> MFRLTAASQKNLNSWYTKGTMRGGVPRIYYAWMRPGSFTRRRFEKMRNPFVDLETGTSLYFRDTRDSAEAIAHAADSKGIKGMDNAIDLYNEYRIVPDLYPEGFQWKHKLNTEYNQWRSNTWLTPDLIPKEHRGRFLCNFQLNIVAYDMRVVKFSPKDHRQWIYCVLYVGSGKGIAGWGRAVAPSTQEAKKEAIREAFSNIIAVDLEQEGPMYPVRVNADGVRVLLYPARRIVANFRVADILCAFGFQHAGCRINLKATNNPKSPTHTVEGVFEAVKALRSVSEIAASRGKVPHSLIYNIYPYLEEIRRRKGMMAMHPPGKDGLLMPDRVVDNRLPDHLKRGYYDDVYWKDFFAGSDEHLNEPRMGLRGDEMRRRLEEAQTSPAPTTAKDTRRRTLEDVLKRLGKTTRDLGSIPIVNPRVDVGLPTHIKRNYQLH;> MVFYSFVLVMKPRQRRFTSQALREIGVAVYSNGGLIRSITNEGIMRPYSRFRDADNTPLTYARYIILQLDMGEEEMGKVDKIIREHQDVLMALKLNNLERPVGIRSGNKELQAAYFPLDTFTRLEEEINWSPQTSADIYTQLEMNWKEFSRTRWSSFLRN;> MLRQSLLSLAKVYGAVPPLGAAQGHRLLHGKREREGSLFAVANDVKRDERLLRQQLNALLEEERMPMQARLQRNEAVSSHEAVPQTPLVDLPGVERRRDLPADPITRLFFQHKGDHALYYGTYDKPSVQDDDRVQIEKRVPRRREENLYTPIYDFCHRIREATEQRKRFVVVPSTIETRGCARVMHDHGLVAGFRDFHNDRAFAVELKYFQGDSTINVIEPCSYDGRTEFEWSPKMMRRLLNTHGIHNRLVVYICRTADNRIIDHIHAVKENIGGRGLMMVH;> MMRKSVTFLRRGKPRPRAGMFPDKYRRVPMLLKPQQGGQQYFNHFLIRSTNDRLTQQDVDNASGQAHSFISPQLPQMDWRNMSARSSEESIREEMRQLAENDVMQHQRVFNERMWYEKEEEHRMKARSCPEETSEHAISNDGAVPPPRVLGGDYFKTRFGYSLVKNSEMTQGPVDYSQLDMWGEMPRYTSDMVFLYLVSRRRNTYAVAYTYEGKRILNTYTAGNRGLKGGDRGFRSEGSTDNGHQVTSMYLNDLLPKLREMRASEGRPMGRGEKVELVVRVMGFYNGRQGAVRAVQDRANEFHVRYFEDITPFPLNGPKMPRGVFK;> MFVRSFCFLRKYGSKSKTPDLKTSFTKTTNFRKAEKISITTTDGEIVKGRGKIRRRTHSALKEAIGAMEHPAIWLWYPWRMNPEPPTPHMPQRRALKNVHGAVFNDLTPVQKKRQEQMLYGVNIPETRQMKFEEQHPLLAGALRKLEGQPKGFPFWYRKYPTRRHAYEYRFSIPVEMLDGYNDDVKKALSKGMMSIQEKQFAQEAMYMERYAEHDFDTTSPAVLAVKRALKCRVLRNHLLTNPHNNIIKTVLANTERKLNHALRRLRKVDFKKYWEIIRDHDVQDILQPPNLVTYRQGSYWKYDWNAGLAISTNLADVMDPRGLNGCVETGRSRSEVARDLGLSYTRPLHENEKKQLSHQAVYYERLAKFKMEQPEAARAMERERFVRKFSGMFVKMDIRSGAPDFPSTYRRLLGTKVVRWASKRHGPN;> MQVTETVLARAVIKRRSPQLWGAPGAPIIRMRGHHVVWKFQSYDLVVEHTHKRRNSDIRLLHYLGKHCPHPQKSLWSPDTPVAQDRHLFMLTTVDIDAFKYWFGVKRCRLSMKPWALLAKAGLLPPSLTQNSKIMPKPLFDKESLMRYYLANRKDEDVMAREKYLNYENSMVKTEEERAAERPVAPYL;> MLRRSLLAFPWWNFQTEHRQRCVLMYGGARTKNTHNANHRVFIKKYKRNAFPNRTRHHWAVSMTGVLSQRPRRMPWPYDLTSLIFNQPRQGSDKIGYVVGTSMLKTAVVATNHMVYYPKFNQRVSRTKRFFAHDEDLACVEGDLVHIKQCRKISKYKHYYVFSILEPNVEGRERLKLGLKAVPPPLFGYPVSRRIVKLNLTSTEGTQEKLAAAIQEHVQDAYRFSGPTPDQPRNRLADPVTFEDANNMIAPNAPAAAALDASDSPPLLDRGEYTEVEQDTRNKKGDDYWMNLQPKEKYDFKSFKKSPRPLEDQVDPRLIDGKYDIPTTASENLYFQ;> MNRTGGSIYAHALSQFAVCRQPWNEYIGLLTKQDSTPYHTEPQEKPAYRGRKQGREGWLFGQQVQLHYHRFPDEQLITNLSRWRTGETVGDIAMQQFRNAQPFDIEDKDPQGVQRPSPEVYMKLNYKNPATISRFLTRTGHMYPADILPLNPEAVVKLRVAKAQAIRIGLYPRFGNPFWFRSQKFRPKAYQENYDPTTYSTKRTVEHFAYNWVQTDRIRRYFRELEAVHTSGSASARGSGGGTTAEHKQQDQFYSPENQPISLHRNNISYMEDVGRSVKNPTVPGLMSTKGMKKKFHNLYSSTSTKRMGFSNPTLGIKKV;> MLRRAYIQRRYPFNKRGPREHKSWKHHVLTEPPKPLQWRDPKVWTRDLSVMKSFDAPQWDLWQSRPRSEDMDEALQPFMDMPKSLKDRRYDIPWWANPFGAWYLQNILSLELLKLKSKTNAEKIATYRSYMRSLASGKDNTMSDDDVIRNIIKERWKTLEFGDRNAGYPCTFGDYIQFLNEWFKSLDEEGMQRLREHFDRRIRPLLAVMSPVDILWLEALTQNSPHNKEQLQRKIAFQTSLGTPEFFDMSKRLRYEINEDYKVRDELGPELFALWSKAPERWPPERLSKMYGLDFTLVRKILVWHHFKACYDACVEPDWSLPKRLFALEWIRDVRARKHGLFYGKMRFAEQKITFYSDRFLFRDLVNRREASYANVWEMDDPYRFLQTEQDYEDYWGDNYDVYRRMFPEMIGRTGEPVQQYGQMPIWAGPHRQHANKSEHNWMFAEIGVNVGHEALKKLELDPTNEKRRRFVIRQPDGTLRSAKMSEMRAWYWKEEWADFRFWAPQMEWGIENTPSQEQYQEHVPDTTDADFRKQRRIQSRPVKWFYESHYTRTGSFAGFQPLRFMQRRTEREVRWPDVINAAVQIQKRKPAAYIFKAIPEL;> MRQCVVRRYKMPKNMGVAPRFDTWNEKYEPWEHMKRMGRLVGTGFYIPPEWYNHFRMFPPINHNFQQEKTLNPHNASEPTQDDTSTLSPERVALRDELARKSRLVASEGMRYYNIFWVRKPLDTMEKEYYELKRRGVDHGEAIRKVLQGFYSGLAVKKRVAAIQAEEAKLTGRFITMREATVVLGVLAKLHKEQLTPHQVSLLAKEQGETTQSGAKLTAIVSRTQPHVNKEASSPATSEAVGSSTEESLSADALASMLSEDGEQSAVGTRYQVEVKETANDSVRQLREKAEDQTGFPDWYTGESPTYSGTS;> MMRSSSFCRRQIRPYYNLPSKSEHGRKMTGFLTPYRHWMWKQNELWRNVHEAQFEHLRRVYKRQWLESFRVNADEYIYKYNITKAAQLAQWECEMKEQEKKRIEARQMMDGRQALKKKHLDLLREFHERQFFFWYERASERLQNMNLINYVPHAQLREHIDKELDKYVAGKNEPYPLNFVGQMPFLEDGDGNIVEVPESLLSNHMAEHPDSTAKPHEPHTSSSISEAAAFEERMLRAMVSAKEEDLKEWLGDDSRALSETIDDISREEEEREADIRVARSMEETDAEREVSRRAYIERGKTGSRSIFRPPTVSEGAGGTPSAPAGDANTPMRRRKKGKLDRVHALQAHQDELLAKLSSQGLKEGVDASSVPERGKIVQSRGRIRDKAVIPTHEVLMQKPELAAGSTPGARIQTKDMVDKMYHRGKYKKSGSGDKSDGEDL;> MLRCARVALRADPLNGGSSMTLGSKGSKLSPEPHRRRMPWTAAKEYVPGVVLNARDKMVLDGVQLLDIESIDRASQLDPLEVLRAVVATREYNISTGKNIFQLASQATYNGRGQRFYRKEWQEGTYDKYVTLSAIDFDRDGNKGTAYGYITFHGETTTRPVQVDFADVPGWYMDFVEERAVPFTGIVPPPPSIGTDVPVDPHSYRLKAYPYYDAPNPPEFVERLLKDRGVLPDTPTETADVDKDPTTSDGSVHYDGK;> MRAGCVACSRIPKLGIAALGSTTTSMQATCQETQELRCATTQMAPAVIFPLPPPLRGSYIDRKPTAASFNEHHATASFRHHMIASADVSHRPRHFYFASGTRNDTGTRSVKEGERKQLKQQTNVEVDSVAYGDQLDELSARWAAKFYGQVTFGPRNYPYPSSRWLARRFQMKKHRIIKRFRFRRYKLAAVANLPFAKMIRVGMLPELKSSKTKRGDVVDPTLSGQLVSAVKNTGEKRKGQRTRPKSKYQV;> MLKRTLTVLDQTYGPHKSYKYTYMPDPRKLAPIETTQRSEIVPQSIRPPTSYVPNHETFLERADIHRLRPTSDFKASFKDWNDLFTCDKRQLRVRGIPRMTRDAIRTAVQAFQNGNPPERFDTKEEWLYYKQFKTVDYSYRVIPELPEKYRPHQSGIDQAPLPDYREINKMPQWAECEERRQSKKTV;> MLRCTVVGHHRSGKARAFVFRDPSLRMMRAGSGYQQLRRMGMPMQVGMGWRKVDSFHANTQYQHAWPLLSHDDLGNSDQSNNTKNIMYSMYMPKRNKGTAPWFRGADTYSVKYCEQGRYEYQRYLMINRFPSEYKKHFLSFLSNIRMSSGSATIPQEALHWLLRMIVDNFNPQHVHYIAAMKTLQSAGELDMARDVWKIMERQQTWPCTATICAYLDVCVEAGEKTWAMEAWNRYCTELKFLEPGEVDPKPISRVPFSLTREELLYLPKWKKHFDHDPNLDVMDLNRFNRTREVYLRMAQVMLAGGERNAFQHFFTKLEEAMLNKPTPVPEPPNPHLVRRPRWAPYEHCKSVHHSPWRLQNNGRALALGPPVTIEDEMQSRFFSNDQFLVHSVKEVLRIVLQEHKRAHPTECTRCKTEAFFYKTKDADETLKFCDDLIERLFASLGVRLSNLNTSSLLSTILEVFRVVGKESGAALLQRANEFLERKASLGDAEGSRENLTASNYLQVLSGFADESAFVYNTKKDGTCQYKTGFDPRTTMRHLADVVQEIAGNPHVTWAADMHLQVVETMVGCGTMKANDYFVRNVLRQFSWDSRFLEALYVEYRRQDDVDMWAELTKRALVWTARYNAPASERLRRLIEDDYDTIRVQTRTFRELAVFQFRDVEERRHSRDVVNELPNPWYDYVAHALPFPDRDAGYPDEYGDLGQWRAPGGPGSPVRGPGYYAPPMEGEHQRGYTAEWRDLRNPMRPPEFPTPWERKYRQYARGQHPSYDMVYAGPMPEIFPMRRDFRKPTRWDFHDIEKQGKYRTSGPY;> MRKFCHFMANCWNSARSHATYGAVPLTHSQVTSVYATDGGKVDELGLLELVEERIFSWKLNKWEMRIPPNLPNDQKELIRQEQENLKQILSEWRKCFGALNADILQISSLTGVPKDVVREKNRTWLQEEVAKLRWMGEVNKAALLRDAFMRLEAFGSRDFMFMERLCCIYGLARQGTFDEAFTNYITEDPVTNDIFVDERNPFKELVAHIVRNYSQIDIIYDFLGFNYSEGYRSSLRRYMEYLQCKTAENVRASGRLVTGDKGEHNILFDYCVSRESLVSGDSCQGIIDFLYINGNDVTLIIIASDNPWLRNRQLPHRRQMEGIARRVCFVLGIPPSEVRIRNLLLPPTYLDKGSIVRLNDIVFRLSNEQSNLLIPWLTNYNKELDPKDVDYTALAKTTNEEEWLTL;> MRCSCAFLDKSVFAAKRRVIVPIHPTPNFPAHFIKSAFTTDPLKEKQKARFSSGGEAMREVQDIPKNLEGERSRRDLASRGDTEFQALVEFIEGASYDQLISGRRFKKVYDVLSENDDMFIWLCHTAMSVLNPGDMRSRLIYNHLRILAESVASGEMTQRTAFRFFESAVRSPAYREIAKRQLEGGAATRLAGISAAADVMRRMGLTRRPMSSYFELYQRIVERSEAMTPWGFPPLFQFEERLSLEPRLKFFSRASQQSLERRRRGHVMTPHTTLHGRRIFWIPPTWNRAGRFLGPHVTLYPGMTPD;> MRRFCTARVSSYVKRAPLLLPRGGRRWRSGAGTTADGGGEKEYIADSFESTAGSNAYAAMELAAEARREIHELWLSAETALEREKRVQQVAALIEKYKLDPSTPREADVSRGLGDAFDRLLLLCLPLGKTDAKGTDNLERLMHLAGRNGRELSVRTIQHLFARTDSFAEALAVFYTMRRCHVAMNMEAYYSMLYSLQRLEEEGWGQHFRNEYEENGAPSEQAMDFIVKGISNALLPENKPWLGRVMFQDRNVPDRRYDTRDFDELDTAWTQRYKSGTPAGAH;> MLHGTPVRRASLRYRRPYWMMFLKGVDNWKIYTVIQQPDHQRTEMLYQAWLGGLDRPYTRPKCMANQPLWLSKKRHMLRKERLDGPETPLEKYVLEWHKKFHSFQGTERPTPDDLHTALDLVERPLDLSYALQLLGQCRNLNNIRFAKETFLVFLEACLRVGRRDCAEYALEHAEPLGFWFIDEDHRRYLQGEQTWYKLSPLDNLYYPVEENAKLNEGRKPITRLSPATESPGSGTAISDGEPSTDVEGETTVDDEIAQLEAELAALEREGGGK;> MFSESLCILSRRFRYNTKFPALVSYNKLPWEVVNHETPQFHMHVAPHYEQLLTLAASSPVPHIIGSKHIDVPREHRLRLLPGMLYLLDGDTLPGEFTINRVLDPTALQYYGRLSSQIVTVEAVRMLVPDDLRLLCNCITFKGPLHLPVAPYASLASLRGASQGGTTGSETGSNCFTLYHFVRPNRPPKELQLEKYYIHAPCVAPLSEFASNSDERGNWRPRLQAPKRTRRATPLPAYRPPQSYLMGLAERLAVVPGGCFGRRSLMWGHWF;> MRRGALSLLKAGLLGHYQQEAFEARKRFEESTTYPGPIRAATPGDTRFYSGSLESILHDTDRHYWRAVTDDPRVQHLIPLRIRFKIFTWVTSGWEQRMQVVQIMAPKDSTIAQVKDLVIVENQSPYLCVSSFHLAIDGKELDPQKTLGEYGITEQSQIDAIEQNDHLLHRDDERPRDWTVDEITAEDVKRSPYKEMEMQPLQNLAPRYEARPKGYFGRTYYSGMKQSS;> MLRRSILFRMKYADLELTTRGEFPHGMKEPAFVKKLDQNIPWYFSTYRSMYHWPITGDNWSDLNEAEKHHDLHMFYTLAWWKLGEGIFGVDEDS;> MFFRFHSTTLQTCLTSGVARSSVAVAVPLRAGCTRREMSSGGDGVLEGAMHKPGESGLQAGSSTTIAGKETWSQFSTKMRYGRRRIRVIDVAAKMSYEYQMLRKMCKRRPAMRQWAVRDDFCDMNPGVVIMSPSMQAAFMKVFRMKEKGLIRQCLRDIVPVIEYRNREEPARLPTNPADMIPEGEPDTLNQKKRELFERREKGENFADLRLHDKRSQAKLRFRIRQRLLKFQRQLAVANAIASRSVLYSTNDAIGYFLFRGAAMYAGMHRVFFELSKQLPHFVPKTMLDFGAGTGTAILVAKEVYDPGSLAYPLYRSLRQTMQGNDSSRTHQLSELRYDLKRLQRNNEEKKKVRFMAVAALLERGEVDPADLPEDLKREIAEVATAAATAKKDRLVREAHARYRDVVDGTEWESGDPLGEVRASTEDPEDVIDGEQGDGGDDGEAAKGRPKTWWEKLIDVENETARTRAARRLRPLQEVTAVEPSPGMMEIGTMVLHDDVPNVTWKRYLLPEDEAIQHDLVVAAYSLSEIATSENRRRIVQQLWKMTKGVLVFVEFANLNNFNILMEARDWILEEKDVGLWDWQPTIVAPCPHEHRCPLRHCKTGVKRKRMRICSTEAHYRSTFVEVWARHMPLKVGIEPISYLILARNELVPERAERRREQLKKAEEMKRRERDVKQQQLHEASLAVKDVVFERLSDEALHRVQSSVPQPLTDIDEVREASTSATSTSLLKDLKDGATSTGEIGHMPTDVPRLVKTGNTRHNRLIFPLQFPPATHKFNRAFVDAGYQRQRAITPAEMLVVRQEVEQLQQRVMRAAPKYLRVVRDPRCHGKVQADFCTPEGDLVSGRVYRRFYGDRNRVSAHSTMRWQHIGGWKLLKRIRRGSLFPHNVPLYAVTKHAQIDFPNTLLDTKHSTVEQTAMQYNDPMSLVEMPDDGLTREELKQKRRLQRDVELQKKVEEKLEDIFGVNAKDWKTDDLGGGRLDARREISEQQWADAVRRAKIRTVQHTKNALPFAAKKRAAQRALQVRRRNVRLEMSGNRRR;> MLTPTRRLPKALSPYAQALRHVALRGATAFGPGAKEMELDMLRKGTLPADYRPPVQGRWDDTIERWAYAWQFPAEEEQDDITKSVERNASGMQALLEIGNKLLRSPPSPEPLSGKASKLYPPVGDMSSGNTALLPPNPTYDVLEQDVSELMAEDAVVVTSQPRLRAEELSAKYNVPMAYIDDSSEASNASKSLALVMEDVGLEFTEDGLTVVISALSRQGYGTIGRAIFDFASAMGLGPSAEMYRALMKYASRRGDVNESMALIEEMKGNGITPRIGNWHELMYTFYKAKDYPAVSQIVDNMKMYANIEPNEVTFVLQLKALAKDNSQLNSLPEAIQLFDQMENVYGFIASRPHYDAMMFHLSQSPRPEMRLRCEELAHKMELMGIVWNANTYLNLIRSAQVVGDVAAVEKYLSRMREEGIPASIGHLTWAVQAHVQSMIRIDYDALKEKDESPLPTWLEHLETCFGIYELVVRRGWVMQLPFVNALLRLTCQATILSMERTPDEAETIGRFEEQANKIWNHTFDEWQLQKDVYSYECYIALLAHQQRIDEAEKLFQEMILKKDLSPSRRTYHCMIFMHLSSGEEGGTARALRYLEAMERAGIQVRPSLLKKIVRVNNAAGYKRDMKRRARRIMQAREEYLARKEEGVSFGEGGKEGASNQRADVDAEGNSILEPLAVSPTSTLAWWEKWKRETVSKHELFTEEGADGTPKGETFEEKNEALRMMGITSSFQTKDLVPQPDRQKLLPLIRREEGEIAGSLWAMDGGELSYPKDGGGPQGWGVRLWRERQLVKREYQKVLDGYRPVPQLSTLGNSVRTAGDQLDIERSGAQTPGELSDYRNFPDNRFDGGQLKPESEAAPAVPFSAELVWQGEANDKLSPYKSDEEIALENDNTFFSSLSKETEGKLSIAVKAMQNKEENSVDVRGKGVTRRSKFDYLEKWRDMYRHGTLEVPEGPTLNFGRTPDDHKETMAALVRGWYQRNRKEPASEEELKRWRVDEQRSSETSASRAALKKRKQVRSRHRNK;> MLRGWHPNSSAMQVGMRHITIGGRHSRGGFRQPLGKHPQVKQGTVEGVPRRIPGTTKVTYTNKKGRTFSFSVPVSELTHPQVTLESAAGTWREMDTSFCELGDIEDDMPSPVDECLRGGSSLDKRLIQEVRERFVSFCREYVLMDTSGMKSTILSTELNAGPDYEHYDRRLRRKRHWLAIRHRFEDVRYVIWPDVVEETARGDSAQADVSLTNPSLTAGEMLEALLWLDAASTFCVRKVHPSDLGDKSEFLPLDLQREVEVVACHARRDLDFFDPSATSLEQFTACAALCVNHRVPFSLFFPAQDVCGDASVSTGQCIVANAPSPHTALGAVRIMALISEGSGSDIGKTIMFSDAFGAVTRFGILRGLSRVMSVEAFGCKDALENVNESELCIILHFCAEVREQNAAFFRRYEASEEDSDPQQVSFLAKYQQLSQIALARCKRLLYHPDSPRAQVMSEDGYIPLVELQRHAEGTNKAALIHYNLGIRSAQGMRRVALGAQSSARLAELVSRLEEASARVSGNTLVNDLVHHLSHKAAAGKMSLTLREVNTLLPLLSRMRRESPNGALDARFDRVFNAIDTAIGAAMRHNCTLDELLDLAEGLAACEMVPSALKQVEMVLIRSVMMHECSPMHLRRMLQAMFTLMRTSVPQVLLQSVASRVADYIKEASHMDSSSSNGGGDEKVKNHEECEQLLELLVVLGKCGYGALPGLVTIYWEAQLIDSMQLNPRLRCSYASLLASAAFALKKHDKRAWEGLADESHRLFMEYTRCNKENDIGRFAECVTGLAVLTQIKDNTNSSDVAFLKEYLSATSLELKSCEVIRVQELTDLLGRTLEWSEALGVVAPDVVIQLEKALFVMLENVSHTAPGVGIPDELVTAACCLVDMSSASLELRKAAAGVVGGAIVHAEEALETLRSGAPTQVRPGHSFDVAALASAERENVYKNSILQYCAALQRSGMSTHVEELWS;> MRHTIPFFRRSAFVPAPGSSLLNPRSQRAKVRRMVAAQKAQGENFERQALYAELGGSPSARAPRSKGERSKEATRRVGCEVAERAKHMTDAEWEGVPVDEKHAFAKYMHKVLQEHPTETTEQQRRRYFETTMADVFELDPRKTVRDEYERVKLGLPVHLKNPQYSLGVSQAVYDAADASLFDPENVHRLENAMTHVKQVFADYVHKKREGVSTEAERRMLANLTAELNLETQKHLANMFKYAEMRLRQVKLEERHHQLAEIERLRRMAQQRGGVKGRKGGSRKMSRMERLKRVINRAVGLDIAVAETVLTEMQAQEEFLQFCEVFARLTLGSGFKHTGKDENLSAYIESLRKLYSMDAATLSTLDVVQYYSSKEGAHPVDWAKRWYERALLLPLQSTPEYQKLLQIQQRDESTVKHIKETAGTGHAFACEAEAEVARIKTQKVVNLVEKMFMDPKDKRLESLHEKRLRYLAHMQMERQIRCVRENAKLFDGVENMPEAAQCRELYEKIMEKKTAQCNMTSPPEGEGSAIQSAKTEGDHCEVGPGMFNVYDDAEASSLFEKIREITLRVIRDRRVQSAAATKARMLNRIIRSLKGGERSIAEELRALHQQRKEKMTMRILGIIENDVKTEMEWLQNMEEAERPPLLPIPENMSYVSAADVQAWRELREDDERKAANPFERRRRTFQPELLGQAWSVPNKPLLFWGTGVSAVQQALRHVAEDAERKRQGLLLAPPYPCAENPWGWRLAKDILDDNN;> MYKKALHSFFLKVHPDFFHHNRSQQTVNESSVARLNELLSWAKAFKSGHLQPPPSSSFTLTFYRKPDDNMGNGETRREGSGSPVSSLVGRSMGDGSLSPTIIQSTFELPSNFAPSDNHRGTVERAVNKFLRDLLRRAACIDSVTESISEAEDATAARAEAKPLRRRPRGSQHRGAPTGPKSLLDEAVESMTVQWSLTPAPTLQELIEADQILFSRDLSPLQSAAALSTLQRHLGELNYSAWESMPVIVSNQFSIGDLTGTITIPWDFTPEQFHSFMAHNEKGVARCREVAIQYASTIEQLIAELCTALELDDILVSCSHQDALRLMELLHRNRELLIQYGLSKLTLEVGNRHATRANGVVIINCSLTSEQLRPWLKAISPKLPLQQRLYELSKQMLESTLWHLKEFRTMVEPGGVDAFSNDCTYAERLQWSKELFRIGPSLAPWDWSEMTFVLSPDVDIDWANGLLALPYNFDGDALVRYVEEVQQEAKSRKREELLAASAMQREEEERRRKQQHDEELMVECQEKGERSGDDSPTVAERMRHLYRQTNPHMDEYLASSNSRVDTLPVERPLSHAVTFNSDAEAEDQLKWEGFYAEPYVDQAPTSDIDDMAHTFMLTNRWHREEAAKKMLDQLRGTYGKKSRRFEYQKMGDVLEINNAKVQPKGFPTLTRGIKPGC;> MLSHAVPRLRLAAAAVKAAEWYAAENRRKQKGGDVIREKVDCTAPLWFDDTEQNLLAREQHVRSPAYRELHRPALTNAAMGLYGGEPGFEKAHRVWVDPDRPHIKHIYNQTALARNLRYARYGYFKRDMHLLDVDKLVRHARLLPTPGRLLTDFLYQRVPLPDKSCAALIRYQRQQIEMLEVWGRHASFQCAVEMFERMIVTNIPPVEVGVETHGEMVLCAAACGKWEEGWNVYANRARELEKESPESFILNTFFFDALLTLCVAAGRVSEGIDTLEEVIKRNLRPRGTMLNKAMILYSILGEQMSKHEASRATSEGERSYLCEPEEVEKMGLEVWSLFDFYQLPRTTASIEAYMRMCCAFNKPTLVLKAQGFADASDIRLSIECFHWLVYAIRGVAGFGDYVMDVLSQLRPRGLTPDFVLFTLSFMYCALQRDGELALAIFDQHFVHQNMNPTPEMVLLFIQACSNCEEPTAVMLERSETLIKRLEAVGSSVDLISPIYDQFLELCAHLGAVASGFSALKRIVGFGKPLTTRMINSLLLANSNAISSNGSLSMTEELVGFFTLLKIRPNADTEICVNLCRDAFGESPVVNDFIKVIGESLQGDSEKGEAPQYDEDIPVIQVPPHELRQLRTEWKLSPRDIVLRRFGQHTKPPGKAALDVGSMRGSVIPFGRSPGEQLV;> MMHRTAARLRMPRKPTPYVRKFLEGCPLPETLVDDIAGANLKSMAPFFTTAPRYIVAAESRLSKLFFHHALYPAGGARRPCRVLIVRGGRSVREPSFTINTGGGRGEVGGGSRGYRDPARRAYFYARPSTVGPFYSGNGGVSSNVAKCHSGVGSEGAGLVKRASVDGLLSPLCGVIEAHFAVGGTCNDAVATEGDGTESLTKGGEKLCVTLAGLLSGGHGGLMMDDGNCASNVRAAKRVARLLHDAAHHLSSFFYVHTQLPDSALFVSRPEASIASDGKGDGLLPSHLAREKDNDGRPSVEGVAVFRLAGGLEPTVHFAVGAPLSVLQRGVDGTASRGEKNSAEEGLNSAASTTVLPFGHIQCLLRVRTRGGKHCAAGKEGSEGTSNTPWCNTAGNDDITSNFAASGPQIAGGIVEPWKLGVSLDPKVPFFMRTLTEKRPSFSCGEGYLGTCSRSGDVDGNTVNDVSSSSGGSRTRAPGEVHMNHLLVRNDCETYLLPQRELLLSFHVPEEAEAMCKEQNEERMRRQAALGYGSPSHVFAEGPRTFARVLHGMKANLAAVEEASSTFRQGAAEGISPQVNGGSTTSGSSRVYEVRALPGDVVFVPRGWKYSVERIVGTAIIDAVAASTASPREALRAVFRTAPDPPLPQDVVRCDEGHAGAGEMPGGDSSNAEIVGVEVDAFVLCYKPYPVLSNAQASTYVAANYVHSGIDDFYAKGGNDVYHKYT;> MTGPTRALFLSSGINLGRLRLAEQFSSMNGWQSKEDPAFDAYVKERRRKENYEAFDQRVERGYAAAAKLHKAEIQNAVKRRLKSSGAKFTAETLREMSSAVTERLAWLRDVWAQIDADYRSGDSARQETAAQEISAALRGEPNDYMRWVYETKRELRFAGPVGRRAIQEELQAAELPEVLDEEVNRYHDLKLNMMEIEREVKAKYGVAGQQHWAELQAAKDEEYIQKLDEAAEVYKQLLDQSARLDESRRSELQRSYVERVHQAQVRFKAAMELEGQREQLIEAHQAMKEERMRTEREKRRQLLREAAELRAQGKKSADVLTALKERQLDANAKRQAEYELKECEDILKRKSEMLDMIAHFKHDVEEREGREMLQRQKSDEERQVNVFGFYEEVGVEDGLSISSEGTTSQGGSSGLGTVSTSTSCAKSADSNSSAQPSQKLRKEELWKVINADTYEDPFRTVHQARLDAVKTYDPAYARTFPLNLVLGRKYSRQGAGEMAAGNETDKQILQKGNNILYSFQWGLNNGTVHDLDADGGTDYFMDGAFHVRDKETGDIDWRYEKKRGGPVFRGPKFYRLGAQREAADPGERAMDPTPYTSTPREHKWRSS;> MPSASSGYTFADFLRRLERSPDSHMAPLYHEHRELFVRRHDMFARVISSVTWSKGVALVAAAGYTQAVNVTIYRALLARMLLHNRHVRQCGAGSVVPWSAALRTYSEAIATHGNAVPTRMTLSALRLCTPARQWVAAISLLMLSQANDKLTLPMLIDAAGCCATPAAWEKAMALLGRFHAQSLQVLPDSIQSLRPVGTSASTVDAAAHALLPRSEGPTPEQKHILTVINKVVSAVPWQVALSNEMCRSYLTHLVASTTLRPTEKTASLTTAVQQLPWEAFVTLMKTVTATVQEGSQGVLGSRSTPQLPPPQDGMERGDVAKSLLSNSIIREGVNLLQSEPETAIPFITTILYKLPSAEAAALFLSEATSAYRNSSSAVVAAAIRHPVVVGALLKRCADSNSWYLAASIFKSTSPTAIPCDVASDLVIQMRRANQAPLVVDVLQKYIVPSRTKLTEEAIEAALLCVLVHNRALAKASAVVAGTSPDNRTGKPNGIGVANGVHWISALSWATDLLEEGVESRILQTGTTPSVGGVNHEDPTVLLRKKTLSPRILSLLIYICVNAGSPRGGLFALGYARTVSKTELELSEEITALLYCMMYDRPREAESIIQHAVKKHGEYKGKYLGRLLVASQEAKGSALRNQT;>MRRLSVSFLPFHLIVTTQRRQFGGNSKDGHKGEDKPIERVGEVPPTGPHPFNITSGAEGQISNQQRKAHDAITQLFRDDAQRKALYQKPGRTIGAQTTTAAISTPPNEDEFEGLQPISGDAEPSSITAVEAVEQELLDDAFLYFPPAQQSASGSVATTATNELYVPGQQIIPPGLTRYRVDVQYQGNDFDGWWKSTTRQLFRREVGLDGSITRVPVAEPGTIGNAAGASRGETMGSRYHARTVLEEALAVALDVNTVRVVAGVIPEVGVSVRRLCCHVDVPSHIELQPRTVIQRATMWMEKRQQPLAILSYRRCKNQDFHARHSGLRRVYVYRILNRVAPPLFDAGLQWHVDRHLDVDRMKRFAKALEGTKDFGYFADPKMANALRRAAMSPGGFSTGAVTEENFQPKATGESHRVTRGKAPKVTMEKGPSNLDRAAALPTFNEYGQRVVQPGAHGKEYYRVATNLPTVRTVDRLDVVRQDDEVLIWFVGRSFLRHQIRNMVSVLKAAGHGLWNDLELQQALQSGFEPSRHRFKRERFPTAPAYGLTLWDVEYPDQHRDDYVQFVDSGPYEQVNIARDI[2x];> MKRYRSSVVTRLVRAITLRPDATVDPERYPLGYVPLDGSESVDSVWSLVKSGAFVAPLSKIETIHRAHVGIRYLTQSEYPALSSIDVVGLQTRLKELCSRLLIRRDFWVLDDYNDPELNSSFGIQNMYFDNFKWSQVLWRRFQQYVEEYFPVAEHTHLTYDEYLQLLRSFSHFEQGAKLLPLLPKRYRIHPPFGVPALSRIDMEPLLLYSQWLKNFRGPLKLDAALVIRSGCGAAVFATKLNGVPIVRGVDPNPRAVMSCRKDAQRMGRRFDSISFRVGEMFPDKDDGNGVPNSRKYDIIVFYPDQGCYNLFFTNAIGEYAPVLTGFAGTLEHFFEEAGDYLSDSGVIVLCCTNVYSILKPTEPHPIEYEIKVNRRWVLLDYYDMPVRGKGTLSHTPTDHHYRIPMEMRKCMRSELWVLHKMTSIAHFAHIHNIPGAQPPSCVVSHWRNKAIGKLRRAVLKGQVESSGGDWDDYKKRLVHLLQEQSENDEDDKAQAIRMAMDPNYPKELADRARAAIEKNMDTDKAFHNNVAKAFGDISPRERFDAYLSCYRL;> MKRIVVPHRWSEMNRVEHPPLMMKQLFQGVCGGLRWLETKSLAQYLAVRAIEEGYPSTPGVRKALHVKRAPLQKRRVVQRSTKSATAACSLPTTAAPAQLPLTSSGDALTVTGGLSLQVTKQKRLVSYDVLDCTLGSGYHAGAVLENGGPYTRVVALDCDHDAMHAARDLVEEFGGDRFRFYCCKMSEAKAMFGERSFDAIMIDGGVSDTQLEDPERGFLLDDEGGHRLDMRFGPQMGVGALEYLNTVSQHTLVSSLLAYGLLEYGQAMKMSRAITRRKPFVDSREVLTCIEQAGDELPEGGWRSQGSRRKSPMSWKFLTSLRCIINNEMYELRQGIENALLMLRDDGRLVVFSRLPWEERLVRGTVDDHPHALLSYVEDISIDDVQIYGFTRHAKMWVITRAASSAYALKNTTTLTEEKFRESSVRWLTGMYAGQTHGFPANNFTFENFERKEWVTLRRNGKPPPVDVGLDDK;> MLCHNRLLLVNKQTQKYRTKLRYRFRQPSVVPLRQTLQQRHNTILEVLRRRRINSGDQSPYRYVEERLYSKPSRLDREGVKVNKTYALQGLGDLEPLRYGANFGISEKDALKYETVAEKAKYMEPPIPYSSLAARKLAAGALWPAAPDPEGMISKEVRLLRHESSMSPSARAFSERVAYHLRRSLKACPGHIAEHIDFTQLIIQEVLGSRRSKEIYIVWFTVDPGARFELEPRLHQLNHWVQQLIIKRVKRRPHIPRVTWIYDGGRLERELPRDVKQELQSFVADAATTLESRVKYLKELDTMNQRMKDIPWFMPYLWSKEEKAARQKSMLADLEEVERRKNEHSSGRSAPPRTSPPPQFVR;>MSAIKRSLNVGVVGMGNMGVPIARNLGFKARSAMYLQIHSRALSKAKRVCDDLSVDGATCAMRIHDRYSTMTKWCDVIVLALADVKASRHALLEDNESLIMNARKGQIIVDHTTVDAETSRECAHEAARRGAYFLDAPMSGSPRACFNGQLLLMVGGDAETFQKMLPIFHMYADNVFHMGESGSGTAAKMISQALVASHNAAAAEALSMAHALGIEDQSKLVQVLDASWGSSTMLRRNAPLLQDLIRNPDKTPPTSAVSVDRLLSDLAHLDASLPKRGGEDEPFPVFDAALRSLAAASDAGMGDRDLASVVHYIEAGEAELRNRTHVPLGGEHLTGRTAATAANSSVNETPSTVNGSSEVPNEFGVEDFY[2x];> MTDPVRRDPTEFLRVLRRMSRTTSWQKTMLFASKGRMVGYRLTREHYNTVLFSQSLWGRALEIVRVVRAMQEDKVQPNGATYYYIVNGMGNADHGWNYDFRINRRLEKIQHWRVALEALEACEANGFDSTDTMHNSALITLVIPGFNRWQQASLLLQRMLREDRRMHPTMVKFYHDCLVRNNRPREASSLMRLAAERGVHGYEDKWEADVYKGRPLDSEVMNESEGNGLRRQASSLAFASLMLRGDQRPLPENLQALLEEETTRNIEAERSVPVPFSAGLHATEINSVFRPRVYRQLWYKWQHIANRYRPTAALKRRQLAPRDSPTGIPGFYRI;> MVAKLQHNSAPTTLNFYEKSFQQLSDVQQRQTGLLIGAAVGDAAARALDGYTAEEVAAVAAESGSLQDEDEDPVVFASVT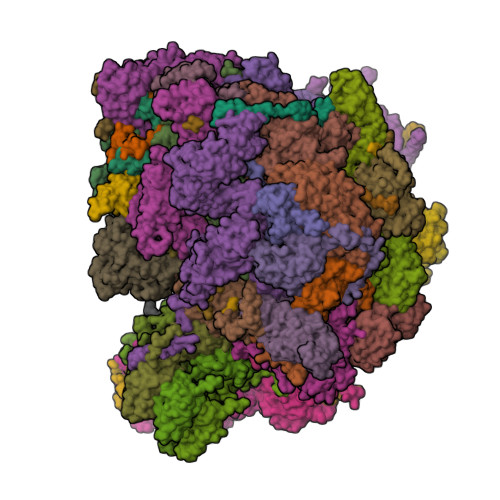PREHKSGLLRHHSYTFYLFSQLLRVMATSRGDFPVQYVKNEWVATARAHPDCFVREHASLLHVLCITMQLPVIYPWADDSTLREYASGFLEFLTETPAEQAVASREDVYAYTNSVLGVALRCLQSNPDPYRNAAFMAAPGTAHVFPDDLALYCPPALVGSSHSRTEELSETDSETVPLFPARLLESDVRVVRECLVVARGAASFAEGIKAAIHLGGPVCQRSLIVGALLGARMGVRRIPISWLSATYDHVPLVTLALQVAQWSWNPPHH;>[5x]MRFINQAASDRAVINAGGRRFETLFSTLHRYPDTPFAQLFPLPGRGARQHRGREFFLDVTPHVFEYILGFLRTNQLNLPAENLQIRAEVVYSMNQWGLLEHAFPPEVIEDGEGCSTGGAVVKLPDVCVVQVCDHMQHDQGVKRHALTITYGADGFQLRSLIRRVRRDLERQLSSTYWQCYQTNERAAFFVTTKVANGTADLLTTSVTQQLVEHTESMGYSLASSYVTLSPDVVHTSVRMLIHNFTFRRSRRVEVEPGDGIALGEGSETIEAEPNIPTMHVGPRREPLNAAESIPPRNERAVNIWTVD;> MSTSSRGILIAGLTNRARTQMAEGILRRLTAGTIFIKSGGVHHESTIHPLAVKVMKDIGIDISKQSVTSLEAARRQQNTYDVYISIDCSYERRTLDKSQPPRAEVRRRESFTVEYGDDGSGPRGGDDPVRYDPLLVPRTPSHWSVGVDATDVRRRWQIWSPRDPSIFHETSTRKFQDHLYEGEPLFMQLRQCPWRTQAKVSERWEMDEVAIRYPVERHSAHELRFVQAREQLLQRSFDLLTKLEKHYGERLLLDRALLEEFIS;> MHPRLSGQGVFPRYGGGWMHQFGHVYALQQELLNAEANNWFRAMELWHTARHEGVAMNVSHYTNILRQCVPPTAWEASLMVLKQMRRENIRPDVVGVGCALAACADANRSEEVEKVFSCFSGKLKLDSICYLALIKAKMSRGGYAEALAVGREQDADGVPFLPHTYTHLLEAAEVADDGEMALELARRMSSEQWPVSDRGREALKKLSTRHHWEEVAEYKQFVAVEDHKLSLPPTLPRG;> MWRLSRSLRSNSLHNPGPFLDGALQLIKLHLAHKNAAADKNTKACSDIEGEFLRELEAFRACFTMSSSLKVAKLYTKKLHGALSYFQLYDDPLMRQLDMIIGKQTMQPSAGRQHGVFKAPVAARLDPFFLDEREETVLPSELPNPPKPDPSTPLRERALKVPAQHRGHWVLRDPDIAITREERRTDPW;> MRRKTTLNIGQVICFSSWNDGSEGYEWKSRALSEKRSLALEFLGNVNKRVSIHDAIRLKADINKKAISNVSCPSFFSGIEGADEDEDQSDMSLCSLLGVLEGEIETDCITHLSPSDASLLKEEFLCDYDPSDTKRMAKWVNLRSETSDYQSYGAIPEGERSLWSAWYLRNIKAGKKPI;> MPPNSATRWLPFVSSDLKDYLNRYWAVMFTVGARPIETGHIRHYVSWYCTRMKVVLLDHHVYVEPLRQQLQEASRTPELPLLFVNKKLVGTLRDVELLEREKKLKDVLHFGFEWRVGGSVAATNGQKSLMGALPAPYGDAEFFRGRYRGPPVARPVVSLPTLHPFALRSEE;> MNCSSTLACHAVVSAPSTASLITSCWTPQQHCYRQLMKSLRAAYFHDRSKLFWSRHRVLVEFYKYSEEANEEAVKQLVAIGLEVAAFIDHHMRTDVERIVKHNETMMALPVAQAKKFRSDYLLAEKQHDSWCKQKIKNIMKRRPPPPYPFF;> MQRSQLARKFATQVGAYSLLRGRCHAVSTWKVMATQAVTIPMYLPVRFHSEGHAAGEEAGRTGQYLLNKDDVLTRVLEVVKNFEKVDASKVTPQSHFVNDLGLNSLDVVEVVFAIEQEFILDIPDHDAEKIQSITDAVEYISQNPMAK;> MRHFGPSIAHFPLSANQLRFKASHIRIANRKRVEMFVAKRFHLPTRLATAAPDIAAEWHDELNPMHMYPAIIGIGHVQPVWWKCAICSHSYQMSVEKRVVRGGGCPQCVVNGKRAVADGALEGEMDSQLRPKRPVMFNMRTKY4-({4-[(2-methylquinolin-6-yl)methyl]piperidin-1-yl}carbonyl)-2-phenylquinoline | C32 H29 N3 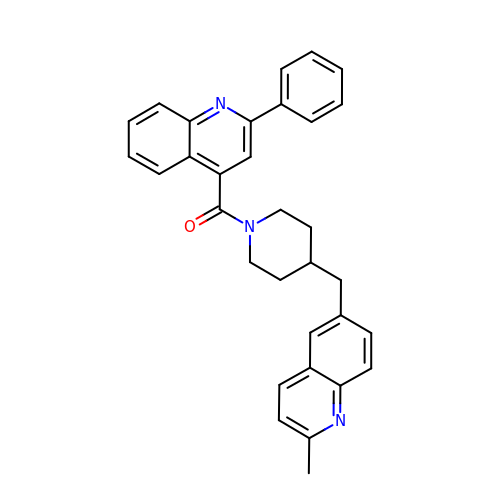O | OZINPIJMBCNUEN-UHFFFAOYSA-N GpsB has emerged as a major regulator of PG biosynthesis in low G+C Gram-positive bacteria, and its homologues (DivIVA/Wag31/antigen 84) in Actinobacteria play essential roles in hyphal growth and branching. To gain molecular understanding of GpsB function, we report three crystal structures of PBP cytoplasmic mini-domains in complex with GpsB, the first structures of a PG synthase in complex with a cytoplasmic cell cycle regulator. The PG synthase arginine finger pokes into a negatively charged cavity situated between α-helices 1 and 2 of GpsB and is fixed in the same orientation in all structures, just as the phosphoryl group defines the binding orientation of peptides to 14-3-345. Therefore, the role of GpsB in the bacterial cell cycle is that of an adaptor, docking PG synthases to other cell wall enzymes, scaffolds and shape determinants into protein complexes for division (the divisome) and peripheral growth (the elongasome).

GpsB is an influential cell cycle regulator in low G+C Gram-positive bacteria and we set out to establish the common rules by which GpsB interacts with major PG synthases in three important bacteria—one model species (B. subtilis) and two pathogens (L. monocytogenes and S. pneumoniae). It has been determined previously by us by SPR that the first 31 amino acids of the cytoplasmic mini-domain of B. subtilis PBP1 (BsPBP1) were critical for binding of BsGpsB19. BsGpsB interacts with the first 16 amino acids of BsPBP1. The backbone amides of BsPBP1Arg8 and BsPBP1Glu9 interact with BsGpsBAsp35, mimicking the mainchain interactions in successive turns in an α-helix. The sidechain of BsPBP1Arg11 forms hydrogen bonds with the carbonyl oxygen of BsGpsBLeu14 and a salt bridge with BsGpsBGlu17. Van der Waals’ interactions connect BsPBP1Arg8 to BsGpsBLeu34 and BsPBP1Glu9 with BsGpsBLys32. BsPBP11-32Arg28Ala had no effect on binding, suggesting that the overall positive charge of the peptide is not the primary determinant of BsGpsB:BsPBP1 interactions, rather the unique physicochemical characteristics of an arginine at position 8 in BsPBP1 is essential. BsPBP11-32Ser7 acts as the helix N-cap, a role that is performed preferentially by Ser, Asn and Thr32, and alanine and proline substitutions in helical positions equivalent to BsPBP11-32Ser7 and BsPBP11-32Ala10, respectively, destabilise model peptides. Finally, the importance of BsPBP11-32Ser7, BsPBP11-32Arg8 and BsPBP11-32Arg11 to GpsB binding is highlighted because these are the most well conserved residues in an alignment of the cytoplasmic mini-domains of Bacillaceae PBP1 PG synthases. The data presented above describe features critical for interactions involving BsGpsB, which include a helical SRxxR(R/K) motif in close proximity to the membrane. In B. subtilis, we discovered a critical motif, SRxxR(R/K), found in close proximity to the membrane that could be used to predict novel GpsB partners.

>[2x]GHMKVKLSAKEILEKEFKTGVRGYKQEDVDKFLDMIIKDYETFHQEIEELQQENLQLKKQLEE;> MSDQFNSREARRKANSK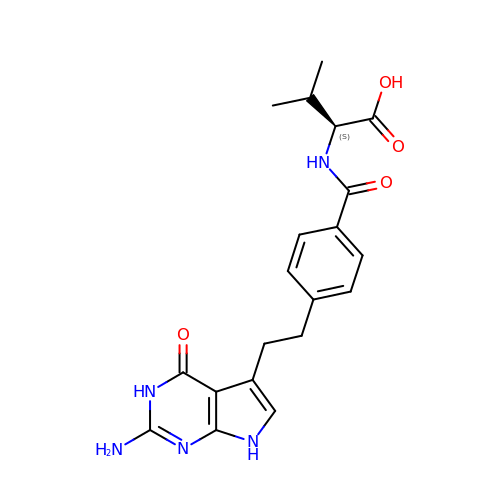2-{4-[2-(2-AMINO-4-OXO-4,7-DIHYDRO-3H-PYRROLO[2,3-D]PYRIMIDIN-5-YL)-ETHYL]-BENZOYLAMINO}-3-METHYL-BUTYRIC ACID | C20 H23 N5 O4 | MYENGRJSPURSQB-HNNXBMFYSA-N> MSSVLKAFERFTIEQELQDRGEEGSIPPETLKSAVKVFVINTPNPTTRYQMLNFCLRIICSQNARASHRVGALITLFSLPSAGMQNHIRLADRSPEAQIERCEIDGFEPGTYRLIPNARANLTANEIAAYALLADDLPPTINNGTPYVHADVEGQPCDEIEQFLDRCYSVLIQAWVMVCKCMTAYDQPAGSADRRFAKYQQQGRLEARYMLQPEAQRLIQTAIRKSLVVRQYLTFELQLARRQGLLSNRYYAMVGDIGKYIENSGLTAFFLTLKYALGTKWSPLSLAAFTGELTKLRSLMMLYRGLGEQARYLALLEAPQIMDFAPGGYPLIFSYAMGVGTVLDVQMRNYTYARPFLNGYYFQIGVETARRQQGTVDNRVADDLGLTPEQRTEVTQLVDRLARGRGAGIPGGPVNPFVPPVQQQQPAAVYEDIPALEESDDDGDEDGGAGFQNGVQLPAVRQGGQTDFRAQPLQDPIQAQLFMPLYPQVSNMPNNQNHQINRIGGLEHQDLLRYNENGDSQQDARGEHVNTFPNNPNQNAQLQVGDWDE

Similar to other mononegaviruses such as Ebola and rabies, MuV uses a single-stranded negative-sense RNA as its genome, which is enwrapped by viral nucleoproteins into the helical nucleocapsid. The nucleocapsid acts as a scaffold for genome condensation and as a template for RNA replication and transcription. Here, we report two MuV nucleoprotein-RNA rings with 13 and 14 protomers, one stacked-ring filament and two nucleocapsids with distinct helical pitches, in dense and hyperdense states, at near-atomic resolutions using cryo-electron microscopy. Structural analysis of these in vitro assemblies indicates that the C-terminal tail of MuV nucleoprotein likely regulates the assembly of helical nucleocapsids, and the C-terminal arm may be relevant for the transition between the dense and hyperdense states of helical nucleocapsids.

The other MuV nucleocapsid with a smaller helical pitch at ~4.5 nm was reconstructed at a final resolution of 3.6 Å. This helical nucleocapsid is also left-handed and contains a twist angle of −26.8° and 13.4 protomers per turn. The rise of this helix is 3.4 Å, which is much smaller than that of NChelix-dense. We described this type of helix as a hyperdense MuV nucleocapsid (denoted as NChelix-hyper). The atomic model of one nucleoprotein from NChelix-dense was fitted into the EM density of NChelix-hyper in a rigid body, and only residues from 1 to 373 were clearly resolved. The C-arm is missing in the NChelix-hyper similar to Nring-13p, Nring-14p, and Nring-stacked. To double check whether NChelix-hyper was formed due to the absence of C-arm, we designed a truncation mutation on MuV nucleoprotein with both the C-arm and the N-tail removed and obtained the pure protein for structural analysis; the truncation mutation assembled into long and hyperdense nucleocapsids (denoted as NChelix-Δarm), which were then examined through a 3D reconstruction. NChelix-Δarm was reconstructed at a resolution at 2.9 Å with almost the same helical rise and twist as NChelix-hyper. Similar tilt transition will occur between NChelix-hyper and Nring-stacked; the tilting angle is ~6.5°. Compared with NChelix-dense, NChelix-hyper has 15% reduction in helical pitch and can reduce the whole length of helical nucleocapsid to 859 nm, which makes it feasible to pack the whole RNA genome in the tiny space of the virion.> MTDLVAVWDVALSDGVHKIEFEHGTTSGKRVVYVDGKEEIRKEWMFKLVGKETFYVGAAKTKATINIDAISGFAY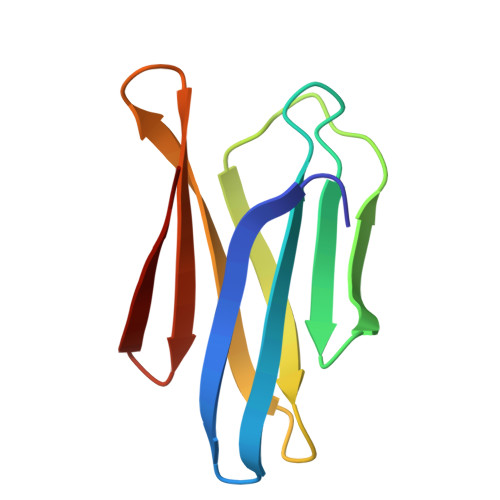EYTLEINGKSLKKYM>PALPEDGGSGAFPPGHFKDPKRLYCKNGGFFLRIHPDGRVDGVREKSDPHIKLQLQAEERGVVSIKGVCANRYL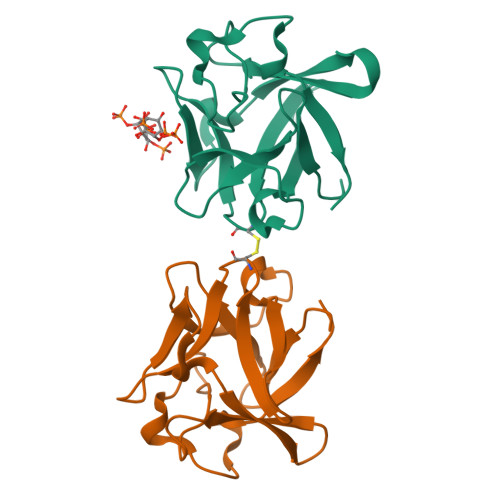AMKEDGRLLASKCVTDECFFFERLESNNYNTYRSRKYTSWYVALKRTGQYKLGSKTGPGQKAILFLPMSAKS[2x]> MGSSHHHHHHSQDPMSMTILPLELIDKCIGSN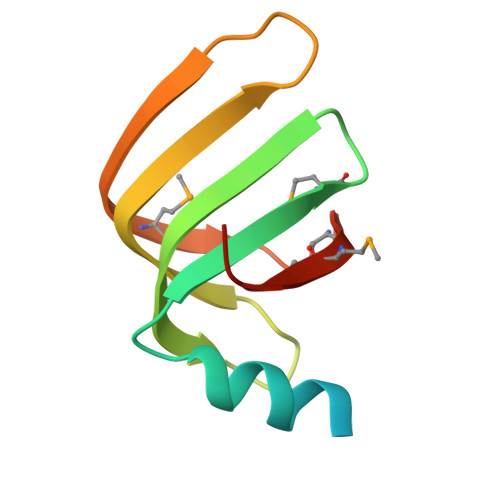LWVIMKSEREFAGTLVGFDDYVNIVLKDVTEYDTVTGVTEKHSEMLLNGNGMCMLIPGGKPE1-hydroxynaphthalene-2-carboxylic acid | C11 H8 O3 | 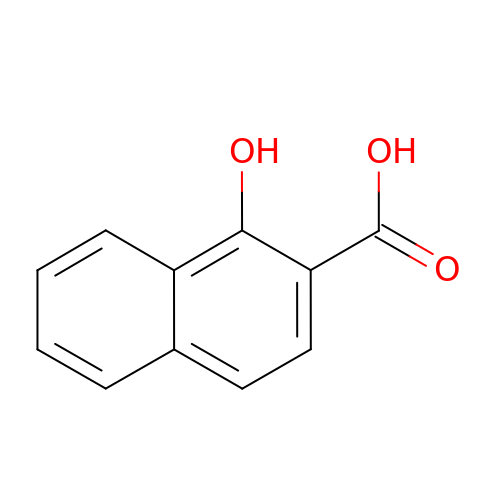SJJCQDRGABAVBB-UHFFFAOYSA-N> GPGSEFRERYELSEKMLSACNLLKYNIKDPKALASKDMRICLNTLQHDWFRVSSQKSAVPAMVGDYIAAFEAVSPDVLRYIINMADGNGNTALHYSVFHSNFQ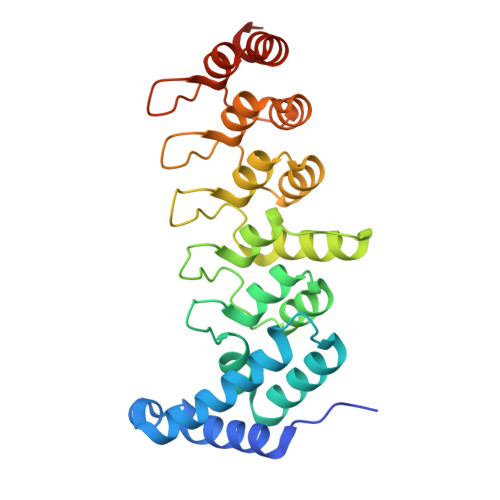IVKLLLDADVCNVDHQNKAGYTPIMLAALAAVEAEKDMQVVEELFSCGDVNAKASQAGQTALMLAVSHGRIDMVKGLLACGADVNIQDDEGSTALMCASEHGHVEIVKLLLAQPGCNGHLEDNDGSTALSIALEAGHKDIAVLLYAHLNFSKAQ> GSPRTVEEIFKDY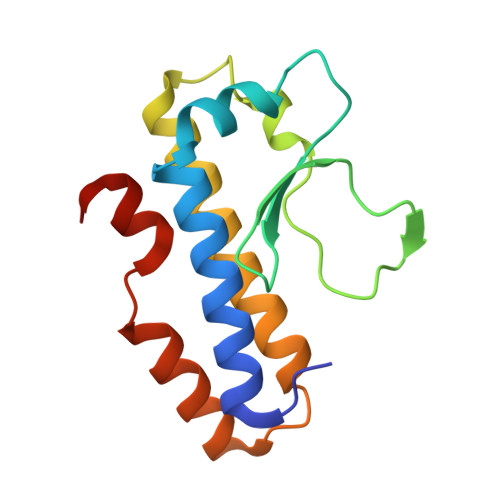SARRAALLRALTKDVDDFYSQCDPEKENLCLYGHPNESWEVNLPAEEVPPELPEPALGINFARDGMQRKDWLSLVAVHSDCWLLSVSFYFGARLNRNERKRLFSLINDLPTLFDVVTGRKAM> PISPIETVPVKLKPGMDGPKVKQWPLTEEKIKALVEICTELEKEGKISKIGPENPYNTPVFAIKKKNSTRWRKLVDFRELNKRTQDFWEVQLGIPHPAGLKKKKSVTVLDVGDAYFSVPLDEDFRKYTAFTIPSINNETPGIRYQYNVLPQGWKGSPAIFQSSMTKILEPFRKQNPDIVIYQYVDDLYVGSDLEIGQHRTKIEELRQHLLRWGLYTPDKKHQKEPPFLWMGYELHPDKWTVQPIVLPEKDSWTVNDIQKLVGKLNWASQIYPGIKVRQLCKLLRGTKALTEVIPLTEEAELELAENREILKEPVHGVYYDPSKDLIAEIQKQGQGQWTYQIYQEPFKNLKTGKYARMR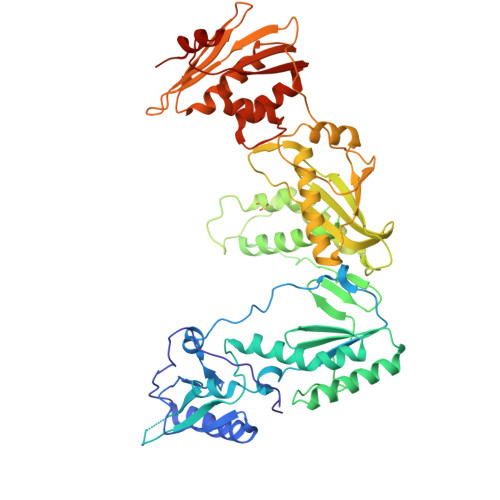GAHTNDVKQLTEAVQKITTESIVIWGKTPKFKLPIQKETWETWWTEYWQATWIPEWEFVNTPPLVKLWYQLEKEPIVGAETFYVDGAANRETKLGKAGYVTNRGRQKVVTLTDTTNQKTELQAIYLALQDSGLEVNIVTDSQYALGIIQAQPDQSESELVNQIIEQLIKKEKVYLAWVPAHKGIGGNEQVDKLVSAGIRKVL> IDITGDWTVAVYCAASPTHAELLELAAEVGAAIAGRGWTLVWGGG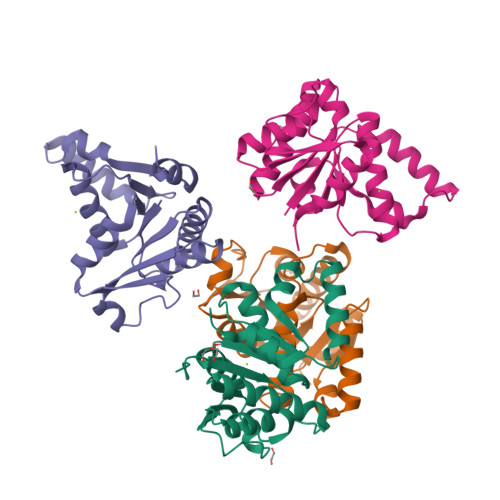HVSAMGAVASAARACGGWTVGVIPKMLVYRELADHDADELIVTDTMWERKQIMEDRSDAFIVLPGGVGTLDELFDAWTDGYLGTHDKPIVMVDPWGHFDGLRAWLNGLLDTGYVSPTAMERLVVVDNVKDALRACAPS;>WTVAVYCAASPTHAELLELAAEVGAAIAGRGWTLVWGGGHVSAMGAVASAARACGGWTVGVIPKMLVYRELADHDADELIVTDTMWERKQIMEDRSDAFIVLPGGVGTLDELFDAWTDGYLGTHDKPIVMVDPWGHFDGLRAWLNGLLDTGYVSPTAMERLVVVDNVKDALRACAPS[3x]>[14x]NLIPTVIEQTNRGERAYDIYSRLLKDRIIMLGSAIDDNVANSIVS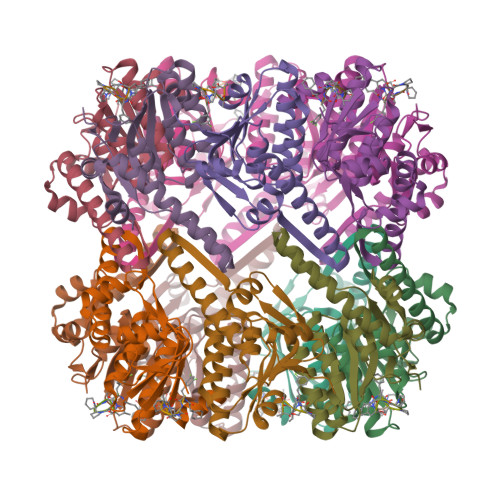QLLFLAAEDPEKEISLYINSPGGSITAGMAIYDTMQFIKPKVSTICIGMAASMGAFLLAAGEKGKRYALPNSEVMIHQPLGGAQGQATEIEIAAKRILLLRDKLNKVLAERTGQPLEVIERDTDRDNFKSAEEALEYGLIDKILTHTEDKKHHH>MPLLVEGRRVRLPQSAGDLVRAHPPLEERARLLRGQSVQQVGPQGLLYVQQRELAVTSPKDGSISILGSDDATTSHIVVLRHTGNGATCLTHCDGTDTKAEVPLIMNSIKSFSDHAQCGRLEVHLVGGFSDDRQLSQKLTHQLLSEFDRQEDDIHLVTLCVTELNDREENENHFPVIYGIAVNIKTAEIYRASFQDRGPEEQLRAA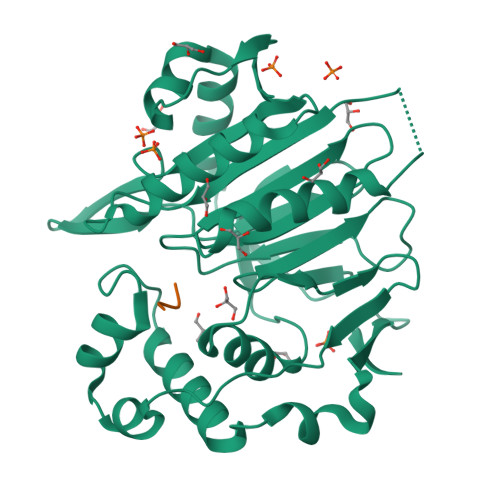RTLAGGPMISIYDAETEQLRIGPYSWTPFPHVDFWLHQDDKQILENLSTSPLAEPPHFVEHIRSTLMFLKKHPSPAHTLFSGNKALLYKKNEDGLWEKISSPGSLEHHHHHH[2x];>[2x]NFAAR> GLPWGCPSDIPGWNTP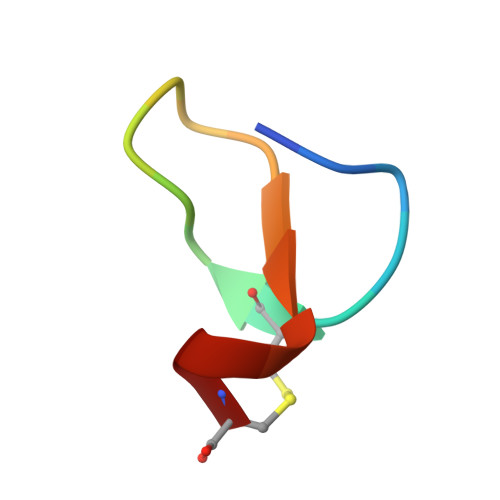WAC>MAGAAAAVTVEEVRKAQRASGPATVLAIGTATPANCVHQADYPDYYFRVTKSDHLTDLKEKFKRMCDKSMIRKRYMHLTEEFLAENPNMCAYMAPSLDARQDIVVVEVPKLGKAAAQKALKEWGQPRSRITHLVFCTTSGVDMPGADYQLTKLLGLRPSVNRLMMYQQGSFAGGTVLRVAKDLAENNRGARVLVVCSEITAVTFRGPSESHLDSLVGQALFGDGAAAVIVGADPDERAERPLFQLVSAAQTLLPDSEGAIDGHLREVGLTFHLLKDVPGLISKNIERALEAAFAPLGISDWNSIFWVAHPGGPAILDQVEAKVSLDKARMRATRHVLAEYGNMSSACVLFILDEMRKRSAED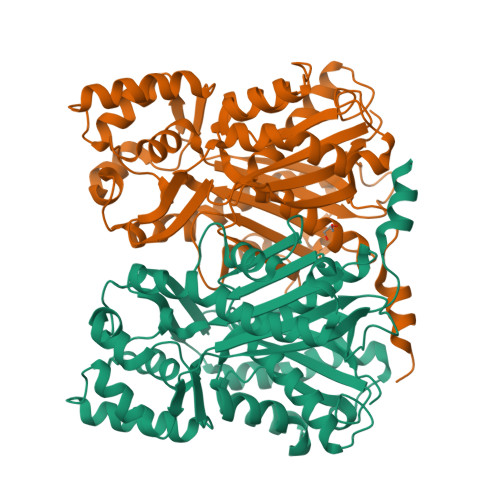GCATTGEGLDWGVLFGFGPGLTVETVVLHSVPITAGAAAA[2x]>MAYTVTNKFQLGFSTLSEELDLESLQVKGTIPKWLSGTLIRNGPAKFEVGKEKFQHWFDGLAMLHKFSFKEGKVSYANKFLESKAYQSARDTDKISYREFATDPCRSIFKRVSSMFSTKFTDNANVNVTKIAERFVAMTETPLPVEFDINTLKTVGVFAYDDKIESGLTTAHPHYDFVKNELVNYATKISRSSNYNVYKIADKTNHRNLIGSIPVEEPAYMHSFAMTENYVVLVEYPFVVKPLDLLLSGKPFIENFSWKPENGTRFIIVNRQNGNLVGTYKSDAFFAFHHVNAFEKQEEIFVDIIAYQDSSIVNALYLDILRGQKTDTIPTSHIRRYRIPLSGGQVEYEMLSSEAV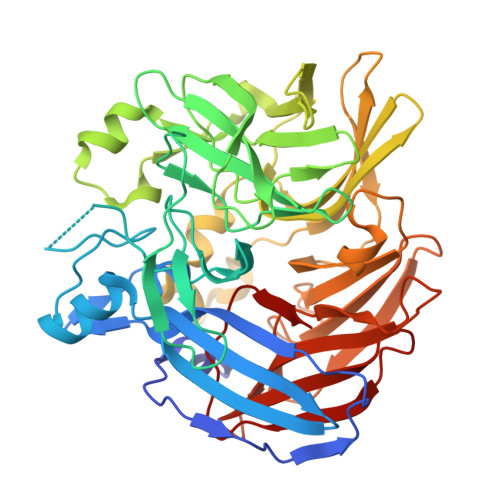ELPRINYKQYNTKDYRFVYGISTYSASDFANQLVKIDILRKSSKIWSEKDCYPGEPVFVGAPDATKEDEGLILSAVLDATNAKSFLLILDATTFEEVARAEVPHHIPFGFHGNYFE[6x]> GIDPFTMATFISVQ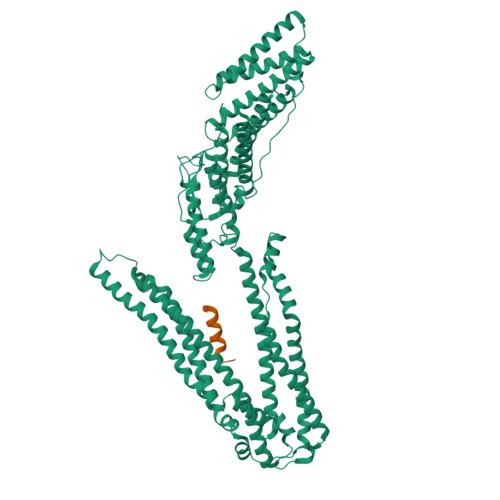LKKTSEVDLAKPLVKFIQQTYPSGGEEQAQYCRAAEELSKLRRAAVGRPLDKHEGALETLLRYYDQICSIEPKFPFSENQICLTFTWKDAFDKGSLFGGSVKLALASLGYEKSCVLFNCAALASQIAAEQNLDNDEGLKIAAKHYQFASGAFLHIKETVLSALSREPTVDISPDTVGTLSLIMLAQAQEVFFLKATRDKMKDAIIAKLANQAADYFGDAFKQCQYKDTLPKEVFPVLAAKHCIMQANAEYHQSILAKQQYYFGEEIARLQHAAELIKTVASRYDEYVNVKDFSDKINRALAAAKKDNDFIYHDRVPDLKDLDPIGKATLVKSTPVNVPISQKFTDLFEKMVPVSVQQSLAAYNQRKADLVNRSIAQMREATTLANGVLASLNLPAAIEDVSGDTVPQSILTKSRSVIEQGGIQTVDQLIKELPELLQRNREILDESLRLLDEEEATDNDLRAKFKERWQRTPSNELYKPLRAEGTNFRTVLDKAVQADGQVKECYQSHRDTIVLLCKPEPELNAAIPSANPAKTMQGSEVVNVLKSLLSNLDEVKKEREGLENDLKSVNFDMTSKFLTALAQDGVINEEALSVTELDRVYGGLTTKVQESLKKQEGLLKNIQVSHQEFSKMKQSNNEANLREEVLKNLATAYDNFVELVANLKEGTKFYNELTEILVRFQNKCSDIVFAR;> SREKPYKEVTEDLLHLNSLF> DLADRFAELERRYDARLGVYVPATGTTAAIEYRADERFAFCSTFKAPLVAAVLHQNPLTHLDKLITYTSDDIRSISPVAQQHVQTGMTIGQ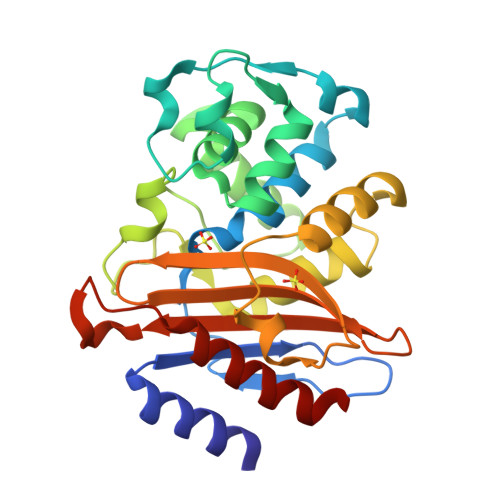LCDAAIRYSDGTAANLLLADLGGPGGGTAAFTGYLRSLGDTVSRLDAEAPELNRDPPGDERDTTTPHAIALVLQQLVLGNALPPDKRALLTDWMARNTTGAKRIRAGFPADWKVIDKTGTGDYGRANDIAVVWSPTGVPYVVAVMSDRAGGGYDAEPREALLAEAATCVAGVLA(S)-5-(1-acetyl-2-cyclopropyl-4-(2-(hydroxymethyl)benzyl)-1,2,3,4-tetrahydroquinoxalin-6-yl)pyrimidine-2-carboxamide 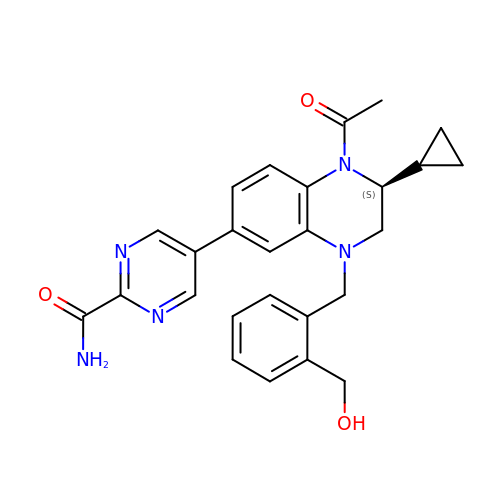| C26 H27 N5 O3 | JVAKWUYUZCOCKR-XMMPIXPASA-N> VVKVYGPAVAVCPQRVMACLLEKGVEFDLVHVDLDSGEQKLPEFLLKQPFGQVPVVEDGDFKLFESRAIIRYYAAKYEDRGPNLLGNTLEEKALVDQWLEIEAH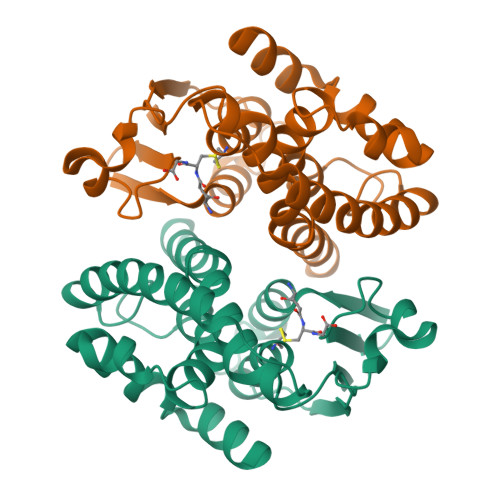NFNDLVFNIVFQVVILPRIGQQGDSELVRTYEEKLEKVLDVYEKRLSKSKYLAGDSFTLADLSHLPATRYLVNEAGLGHLVKDRKKLNAWWEDISSRPAWKKLMNLAGF5-chloro-N~2~-{5-methyl-4-(1-methylpiperidin-4-yl)-2-[(propan-2-yl)oxy]phenyl}-N~4~-{1-methyl-3-[(propan-2-yl)sulfonyl]-1H-pyrazol-4-yl}pyrimidine-2,4-diamine | C27 H38 Cl N7 O3 S | 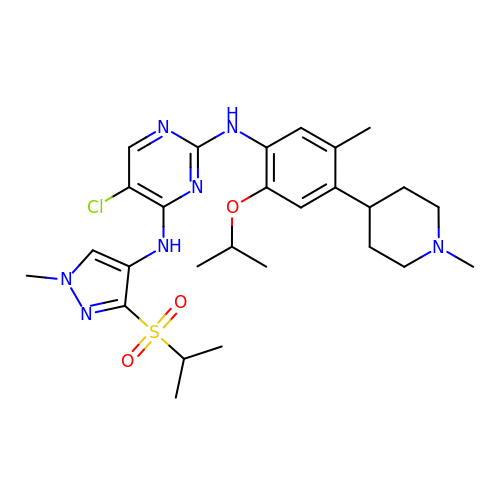CNIWZQPSVDYFSY-UHFFFAOYSA-N>[2x]SADHVNPSSQLSYAELQIYGDMNYVDVHRLYTYAFTQHLMGCWNTTNYGGQHRMDDNEMSRPWNNLYPGAMRNLTDAIEATKDDGTQVNVYAALRIFRVYVGALLTD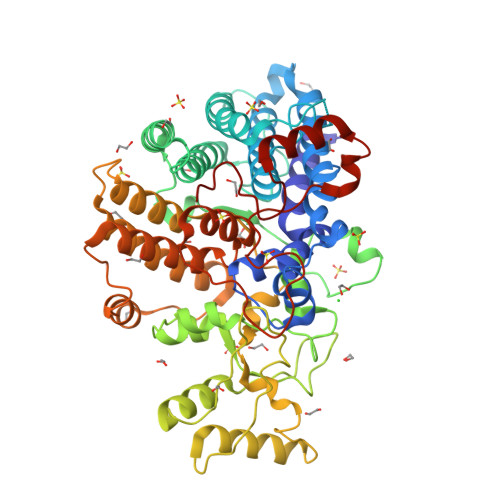YYGDIPFTEAGLGYITGNSKPKYDKQEDLYRFFFSELKEAAGLFDINAKAITSDPLFGGNIAEWITFANSLRLRYAMRLSDVLPDLAKTEFVAALEDGVMVSGTDDACIKHMNVSYSFGQEAYRDIRGNAMAKYFYGNDPANNPSYLCQTFWEQLYKNNDPRTTRLCRFYIDDFMSISTGDGRIDVTDAVLATQAANPSADVIYMIAPGEFSWDNWPSYTDILGSPLATQIAEIQAAHPDYNPGSNPRWLMPKLAGNFLRSDNPGILMTYAEVCFLRAEAAVLGWTADNAKDFYESGIRAAMDLLATYYGCSVVTDAEFAAYIAETSVAFGAVAEQQKSQINTQAWILHFHNPAEAWANVRRADYPKLQAPNTKNPLIDGADIPVRLCYPIKEETYSKDAYQEAKDRVGDYSWHARLWWDVK>DSCMSFQCKRGHICKADQQGKPHCVCQDPVTCPPTKPLDQVCGTDNQTYASSCHLFATKCRLEGTKKGHQLQLDYFGACKSIPTCTDFEVIQFPLRMRDWLKNILMQLYEANSEHAGYLNEKQRNKVKKIYLDEKRLLAGDHPIDLLLRDFKKNYHM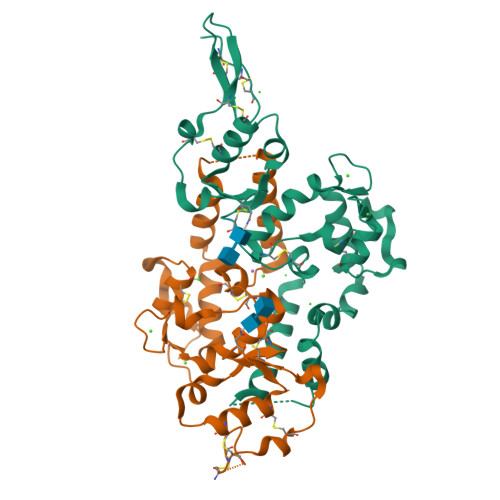YVYPVHWQFSELDQHPMDRVLTHSELAPLRASLVPMEHCITRFFEECDPNKDKHITLKEWGHCFGIKEEDIDENLLFASTSHHHHHH[2x]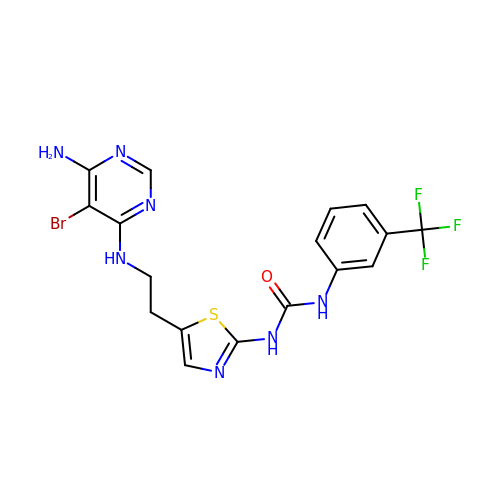1-(5-{2-[(6-amino-5-bromopyrimidin-4-yl)amino]ethyl}-1,3-thiazol-2-yl)-3-[3-(trifluoromethyl)phenyl]urea | C17 H15 Br F3 N7 O S | RLZZNXXMMUZRIT-UHFFFAOYSA-N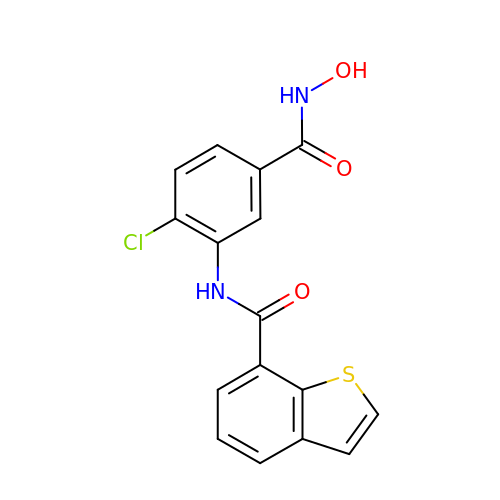~{N}-[2-chloranyl-5-(oxidanylcarbamoyl)phenyl]-1-benzothiophene-7-carboxamide | C16 H11 Cl N2 O3 S | FRUVCGVXUWSDQY-UHFFFAOYSA-N4-{(1S)-1-[(5-chloro-6-{[(5S)-2-oxo-1,3-oxazolidin-5-yl]methoxy}-1H-indole-2-carbonyl)amino]-2-hydroxyethyl}benzoic 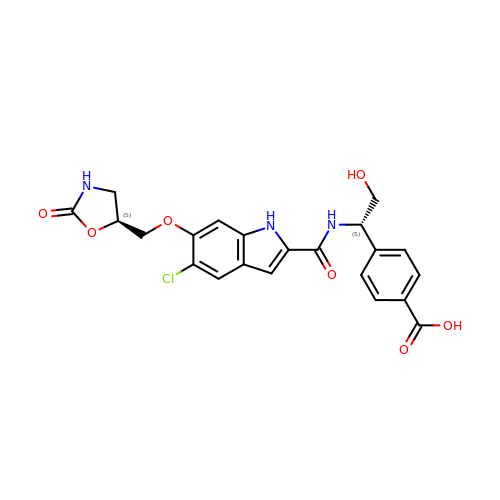acid | C22 H20 Cl N3 O7 | HSLVBDMYOQHSSR-KBXCAEBGSA-N>GSSMSAPTNLEQVLAAGGNTVEMLRNSQIGAYVYPVVAPEFSNWRTEQWAWRNSAVLFDQTHHMVDLYIRGKDALKLLSDTMINSPKGWEPNKAKQYVPVTPYGHVIGDGIIFYLAEEEFVYVGRAPAANWLMYHAQTGGYNVDIVHDDRSPSRPMGKPVQRISWRFQIQGPKAWDVIEKLHGGTLEKLKFFNMAEMNIAGMKIRTLRHGMAGAPGLEIWGPYETQEKARNAILEAGKEFGLIPVGSRAYPSNTLESGWIPSPLPAIYTGDKLKAYREWLPANSYEASGAIGGSFVSSNIEDYYVNPYEIGYGPFVKFDHDFIGRDALEAIDPATQRKKVTLAWNGDDMAKI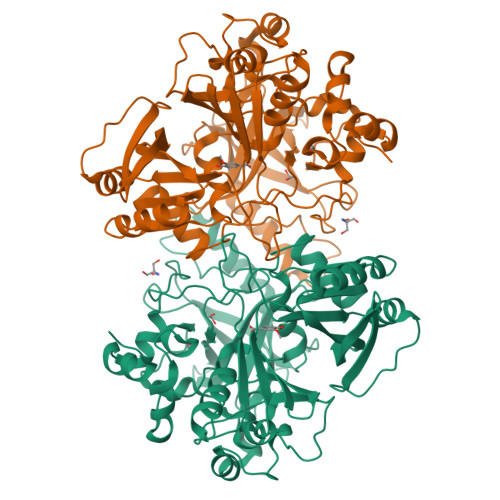YASLFDTEADAHYKFFDLPLANYANTNADAVLDAAGNVVGMSMFTGYSYNEKRALSLATIDHEIPVGTELTVLWGEENGGTRKTTVEPHKQMAVRAVVSPVPYSVTARETYEGGWRKAAVTA[3x]> MPKTPHTKGPDETLSLLADPYRFISRQCQRLGANAFESRFLLKKTNCLKGAKAAEIFYDTTRFEREGAMPVAIQKTLLGQGGVQGLDGETHRHRKQMFMGLMTPERVRALAQLFEAEWRRAVPGW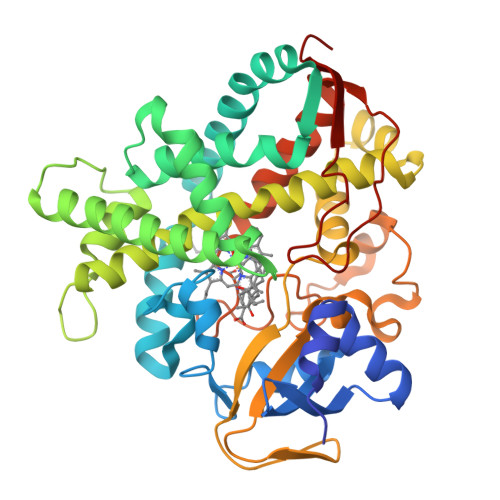TRKGEIVFYDELHEPLTRAVCAWAGVPLPDDEAGNRAGELRALFDAAGSASPRHLWSRLARRRVDAWAKRIIEGIRAGSIGSGSGTAAYAIAWHRDRHDDLLSPHVAAVELVNVLRPTVAIAVYITFVAHALQTCSGIRAALVQQPDYAELFVQEVRRFYPFGPAVVARASQDFEWEGMAFPEGRQVVLDLYGSNHDAATWADPQEFRPERFRAWDEDSFNFIPQGGGDHYLGHRCPGEWIVLAIMKVAAHLLVNAMRYDVPDQDLSIDFARLPALPKSGFVMRNVHIGG>[2x]MEELRKWPLYRAVIAEFVATLLFLYVSILTVIGYKAQTDATAGGVDCGGVGILGIAWAFGGMIFVLVYCTAGISGGHI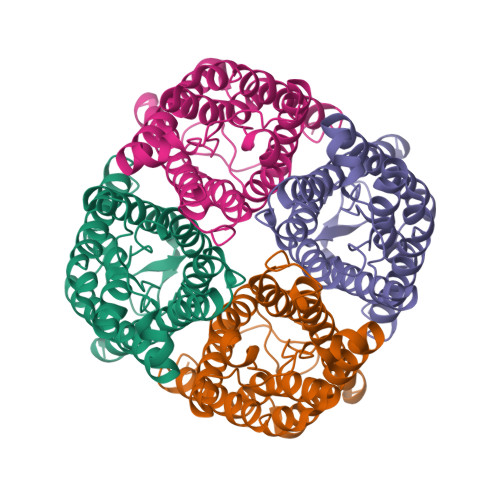NPAVTVGLFLARKVSLVRTVLYIVAQCLGAICGCGFVKAFQSSYYTRYGGGANELADGYNKGTGLGAEIIGTFVLVYTVFSATDPKRNARDSHVPVLAPLPIGFAVFMVHLATIPITGTGINPARSFGAAVIYNNEKAWDDQWIFWVGPMIGAAAAAFYHQFILRAAAIKALGHHHHHHHH> GTDSQLAQWASTRFRSFKRASTLNQQQATLKRKAPVDPNTAFYFNKDPIKESLIEMEAKLSKKAIKNFSEIMMWMGDYPIPKGQTASLVIQSIISRGIENHELRDEIYCQAYRQTNKNPKVESAKKGFELIYFLSITFSPSDSLLQPFMEQLMSRNIAIQSSSPQLASLIAVCIEKLESHPIPSYQQRKMGPSATEIQSFRSNLENGDISTCKIRFIDQSTKLAKINTYTTIREITDTVCRQYGISQQSIKMFGISAVNETAGISKVVSETDMIYDVLARWEQS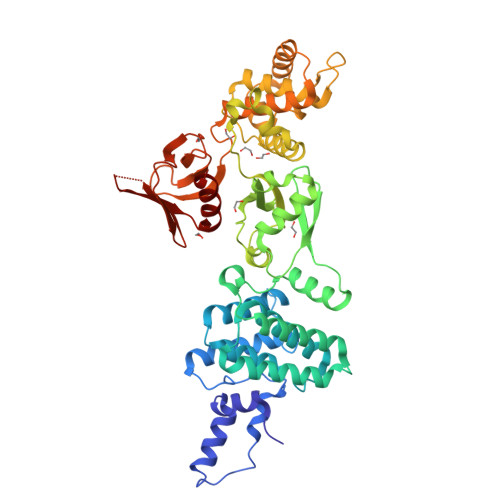EEKGEFYFQVRRRFFLDDVNKILDQEHLWTDDDICFELTYCQIRDEWMKGLYTNVNEKDSSIIAAILIQLLYPNQSKLVLTKEVVRQVLPDQILNSQNIKVWISMIESQIFELVSQTPEYLKLMFINLIGSKSPLFGCTLFNIQQKENPPKAWLAINKKGVSIFDPHTKESKNFWTFQSISNVAFTDDTFCIMTGNLMKPIKQTFTTDEHSSIASVYQFYSSQ N-methyl-L-tryptophan | 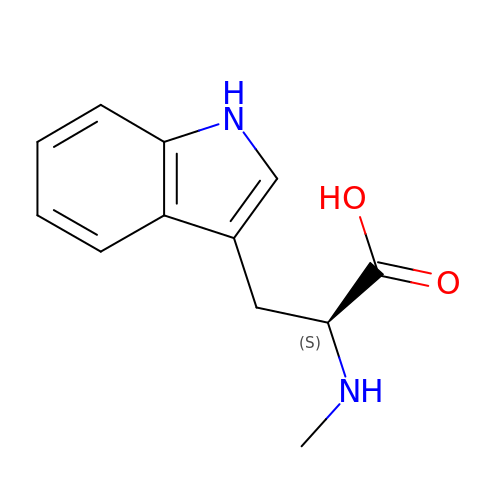C12 H14 N2 O2 | CZCIKBSVHDNIDH-NSHDSACASA-N The protein Pgp3 is implicated in the sexually transmitted disease chlamydia and comprises an extended complex arrangement of a C-terminal domain (CTD) and an N-terminal domain (NTD) linked by a triple-helix coiled coil (THCC). One of these, the Pgp3 protein, is transcribed from the CDS5 gene. This protein is both associated with the bacterial outer membrane and secreted into the cell cytosol, and is thought to be a virulence and in vivo fitness factor supporting Ct infection. X-ray crystallographic studies of Pgp3 from a genotype D strain of Ct have been reported at a resolution limit of 3.1 Å by Galaleldeen et al., establishing that the 84 kDa Pgp3 trimer is comprised of globular N- and C-terminal domains connected by a triple-helical coiled coil (THCC). Recently, Hou et al. reported that Pgp3, specifically its central region, neutralizes the activity of cathelicidin LL-37, an antichlamydial peptide secreted by epithelial cells and neutrophils in the human genital tract.

Here, the X-ray crystal structure of Pgp3 from an LGV1 strain is reported at the highest X-ray diffraction resolution obtained to date for the full protein. The protein was crystallized using a high concentration of potassium bromide, which resulted in a new crystal form with relatively low solvent content that diffracted to a resolution of 1.98 Å. Since the threefold axes of the THCC and NTD are not collinear with the threefold axis of a CTD, this naturally leads to disorder in the THCC and the portion of the NTD that does not directly interact with the CTD via crystal packing. c and anomalous difference electron density derived from diffraction data measured on the high-energy side of the Br K-edge peak to enhance the bromine signal, as well as the local structural environment of each peak, a total of 28 bromide ion-binding sites have been identified in our study. A total of 28 such ions were identified. These are basically all in the CTD. The most common form of interaction is via a hydrogen bond to a peptide NH. Our LGV1 isolate Pgp3 crystal structure shows where amino-acid changes actually occur (Q12E, T39K, P61S, D86N, Q90D, R138S, Y191C, R210S and I212T) compared with the Pgp3 crystal structure reported by Galaleldeen et al.. Of special importance is the lattice interaction that is observed in both crystals involving the three Phe6 residues on the fairly flat NTD surface and one of the Trp234 residues on the curved surface of the CTD.

>MGNSGFYLYNTQNCVFADNIKVGQMTEPLKDQQIILGTTSTPVAAKMTASDGISLTVSNNPSTNASITIGLDAEKAYQLILEKLGDQILQGIADTIVDSTVQDILDKITTDPSLGLLKAFNNFPITNKIQCNGLFTPRNIETLLGGTEIGKFTVTPKSSGSMFLVSADIIASRMEGGVVLALVREGDSKPYAISYGYSSGVPNLCSLRTRIINTGLTPTTYSLRVGGLESGVVWVNALSNGNDILGITNTSNVSFLEVIPQTNA[6x]> MGSDKIHHHHHHENLYFQGMYKVGIVLFDDFTDVDFFLMNDLLGRTSDSWTVRILGTKPEHHSQLGMTVKTDGHVSEVKEQDVVLITSGYRGIPAALQ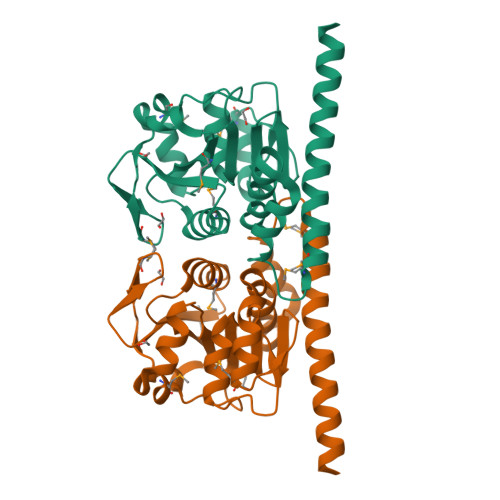DENFMSALKLDPSRQLIGSICAGSFVLHELGLLKGKKLTTNPDAKAVLQGMGGDVQDLPLVIEGNIATAGGCLSLLYLVGWLAERLFDSVKRKQIQNQLIPAGQMEIFETLISETIQSAESAYEYRSACESDAESLVV>MGSSHHHHHHSSGGNENLYFQGHMARASGSERHLLLIYTGGTLGMQSKGGVLVPGPGLVTLLRTLPMFHDKEFAQAQGLPDHALALPPASHGPRVLYTVLECQPLLDSSDMTIDDWIRIAKIIERHYEQYQGFVVI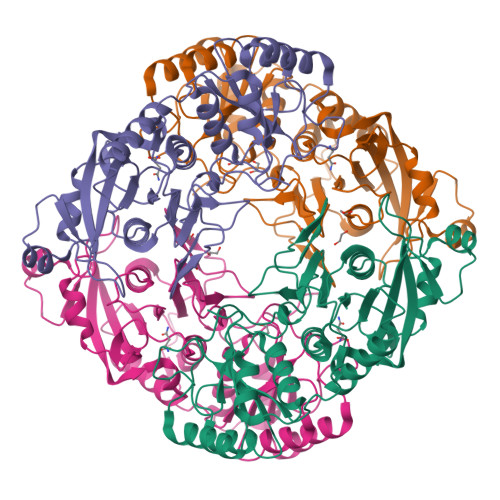HGTDTMASGASMLSFMLENLHKPVILTGAQVPIRVLWNDARENLLGALLVAGQYIIPEVCLFMNSQLFRGNRVTMVDSQKFEAFCSPNLSPLATVGADVTIAWDLVRKVKWKDPLVVHSNMEHDVALLRLYPGIPASLVRAFLQPPLKGVVLETFGSGNGPSKPDLLQELRAAAQRGLIMVNCSQCLRGSVTPGYATSLAGANIVSGLDMTSEAALAKLSYVLGLPELSLERRQELLAKDLRGEMTLPTADLHQSSPPGSTLGQGVARLFSLFGCQEEDSVQDAVMPSLALALAHAGELEALQALMELGSDLRLKDSNGQTLLHVAARNGRDGVVTMLLHRGMDVNARDRDGLSPLLLAVQGRHRECIRLLRKAGACLSPQDLKDAGTELCRLASRADMEGLQAWGQAGADLQQPGYDGRSALCVAEAAGNQEVLALLRNLALVGPEVPPAI[4x]> GMLTKFETKSARVKGLSFHPKRPWILTSLHNGVIQLWDYRMCTLIDKFDEHDGPVRGIDFHKQQPLFVSGGDDYKIKVWNYKLRRCLFTLLGHLDYIRTTFFHHEYPWILSASDDQTIRVWNWQSRTCVCVLTGHNHYVMCAQFHPTEDLVVSASLDQTVRVWDISGLRKKNLSPGAVESDVRGITGVDLF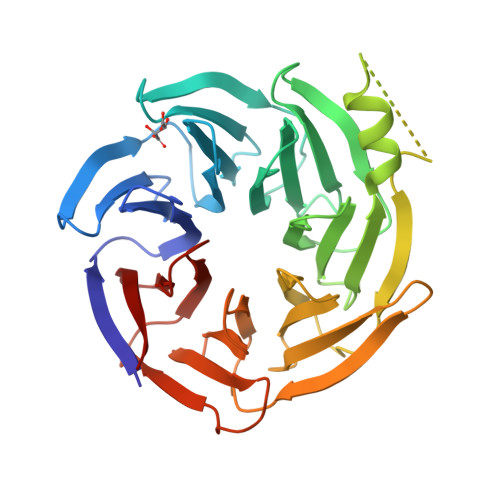GTTDAVVKHVLEGHDRGVNWAAFHPTMPLIVSGADDRQVKIWRMNESKAWEVDTCRGHYNNVSCAVFHPRQELILSNSEDKSIRVWDMSKRTGVQTFRRDHDRFWVLAAHPNLNLFAAGHDGGMIVFKLE>SSTQIGGMSLDQARTQLAPWTQRAAPIGADEYQQRIERARVLMRAQGVDALLIGAGTSLRYFSGVPWGASERLVALLLTTEGDPVLICPAFEEGSLDAVLQLPVRKRLWEEHEDPYALVVQAMDEQHAHALALDPGIAFAVHTGLRAHLGTAIRDAGAIIDGCRMCKSPAELALMQQACDMTLLVQRLAAGIAHEGIGTDQLVRFIDEAHRALGADNGSTFCIVQFGHATAFPHGIPGVQHLRAGELVLIDTGCTVQGYHSDITRTWIYGTPSDAQQRIWELELAAQAAAF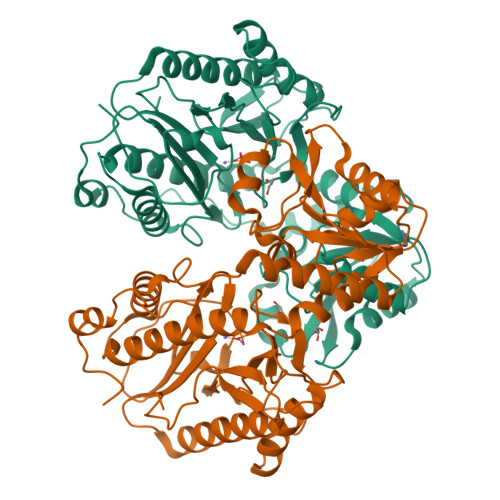AAVRPGVACEAVDQAARAVLQAAGLGPDYRLPGLPHRTGHGCGLAIHEAPYLVRGNRQPLQPGMCASNEPMIVVPGAFGVRLEDHFYVTDTGAQWFTPPSVAIDQPFA[2x];> GGG>GSAPSRKFFVGGNWKMNGRKQSLGELIGTLNAAKVPADTEVVCAPPTAYIDFARQKLDPKIAVAAQNCYKVTNGAFTGEISPGMIKDCGATWVVLGHSERRHVFGDSDELIGQKVAHALAEGLGVIACIGEKLDEREAGITEKVVFEQTKVIADNVKDWSKVVLAYEPVWAIGTGKTATPQQAQEVHEKLRGWLKSNVSDAVAQSTRIIYGGSVTGATCKELASQPDVDGFLVGGASLKPEFVDIINAKQ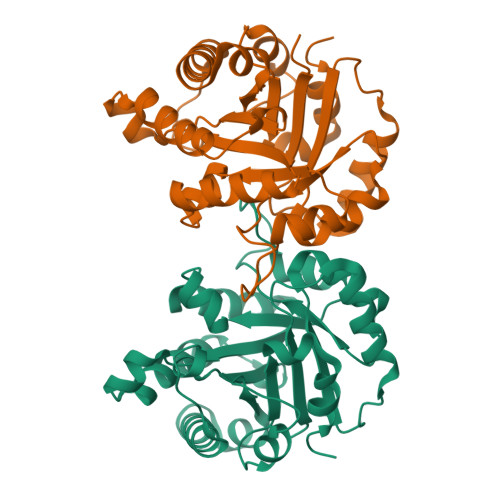[4x]>[3x]VQIGPVTDLHIVNADIVPDGFVRPAVNAGGTFPGPVIAGNVGDNFQIVTFNQLIECSMLVDTSIHWHGEFQKGTNWADGPAFITQCPIIVGNSFSYNFNVPGMAGTYWYHSHLTTQYCDGLRGPFVVYDPNDPDANLYDVDDDTTIITLADWYHVLAKEMGAGGAITADSTLIDGLGRTHVNVAAVPLSV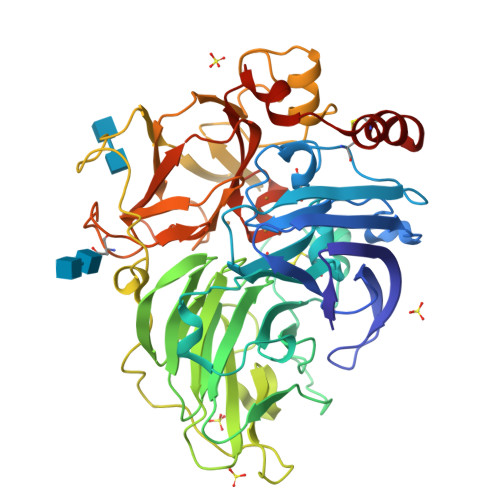ITVEVGKRYRMRLVSISCDPNYDFSIDGHDMTIIETDGVDSQELTVDEIQIFAAQRYSFVLNANQPVGNYWIRANPNSGGEGFDGGINSAILRYDGATTADPVTVASTVHTKCLIETDLHPLSRNGVPGNPHQGGADCNLNLSLGFACGNFVINGVSFTPPTVPVLLQICSGANTAADLLPSGSVISLPSNSTIEIALPAGAAGGPHPFHLHGHDFAVSESASNSTSNYDDPIWRDVVSIGGVGDNVTIRFCTDNPGPWFLHCHIDWHLDAGFAIVFAEDIPNTASANPVPEAWSNLCPSYDSAH> GAMAPLQPGDSFPANVVFSYIPPTGSLDLTVSGRPIEYNASEALAKGTSVLVAVPGAFTPTCQEKHVTGFIAKLDQLRQAGVDRVLFIASNDAFVMSAWGKANGIKDESILFLSDSDTAFSSS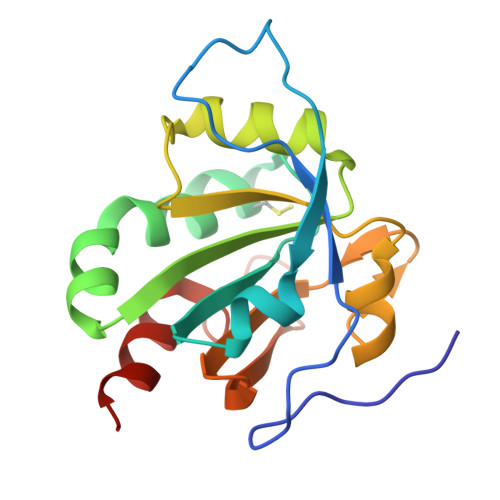IGWANAGRTGRYAIVVKDGKVVYAAVDTVRGSTEKSGVDAVLTVLGNQGKL>[4x]AEIPLKYGATNEGKRQDPAMQKFRDNRLGAFIHWGLYAIPGGEWNGKVYGGAAEWLKSWAKVPADEWLKLMDQWNPTKFDAKK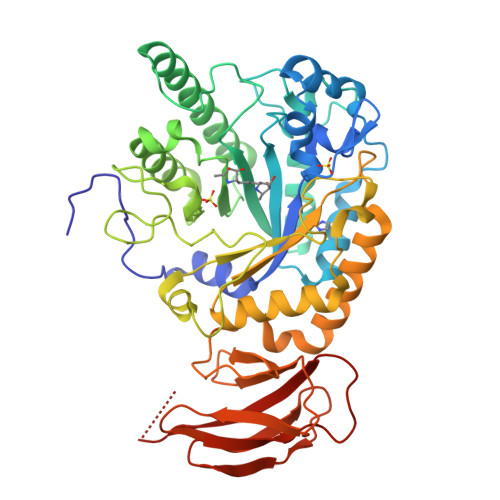WAKMAKEMGTKYVKITTKHHEGFCLWPSKYTKYTVANTPYKRDILGELVKAYNDEGIDVHFYFSVMDWSNPDYRYDIKSKEDSIAFSRFLEFTDNQLKELATRYPTVKDFWFDGTWDASVKKNGWWTAHAEQMLKELVPGVAINSRLRADDKGKRHFDSNGRLMGDYESGYERRLPDPVKDLKVTQWDWEACMTIPENQWGYHKDWSLSYVKTPIEVIDRIVHAVSMGGNMVVNFGPQADGDFRPEEKAMATAIGKWMNRYGKAVYACDYAGFEKQDWGYYTRGKNDEVYMVVFNQPYSERLIVKTPKGITVEKATLLTTGEDITVVETTRNEYNVSVPKKNPGEPYVIQLKVRAAKGTKSIY> MGRGKVKPNRKSTGDNSNVVTMIRAGSYPKVNPTPTWVRAIPFEVSVQSGIAFKVPVGSLFSANFRTDSFTSVTVMSVRA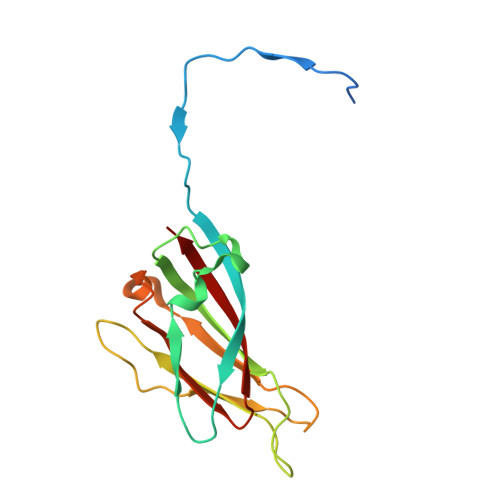WTQLTPPVNEYSFVRLKPLFKTGDSTEEFEGRASNINTRASVGYRIPTNLRQNTVAADNVCEVRSNCRQVALVISCCFN D-SORBITOL-6-PHOSPHATE | C6 H15 O9 P | 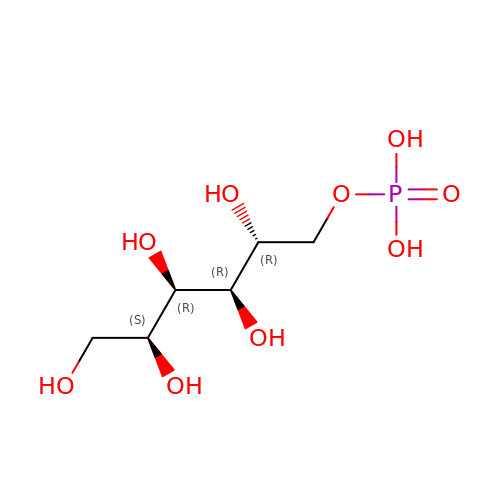GACTWZZMVMUKNG-SLPGGIOYSA-N> TIQPGTGYNNGYFYSYWNDGHGGVTYTNGPGGQFSVNWSNSGEFVGGKGWQPGTKNKVINFSGSYNPNGNSYLS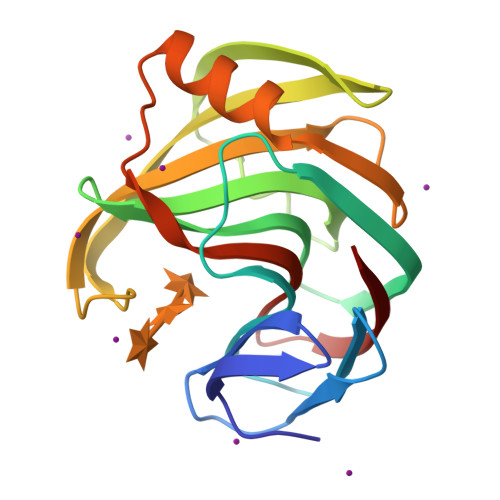VYGWSRNPLIEYYIVENFGTYNPSTGATKLGEVTSDGSVYDIYRTQRVNQPSIIGTATFYQYWSVRRNHRSSGSVNTANHFNAWAQQGLTLGTMDYQIVAVQGYFSSGSASITVS UdgX excises uracil from uracil-containing DNA to concurrently form a covalent bond with the resulting AP-DNA. Structurally, UdgX is highly similar to family-4 UDGs (F4-UDGs). However, UdgX is unique in possessing a flexible R-loop (105KRRIH109). Our earlier studies allowed us to propose a reaction mechanism of UdgX, which involves the formation of a covalent bond between H109 of UdgX with the C1′ position of the target deoxyribose sugar concurrently with the uracil excision from this site in DNA.

Substitutions of His109 in MsmUdgX with Ser, Gly, Ala, Gln, Cys and Lys showed the loss of its covalent complex formation with DNA but gained canonical UDG activities. However, H109 substitutions by Gln or Lys, showed poor activity. Both Cys and Ala mutations of H109 showed intermediate Kcat/Km values. Further, the overlay of all the structures of UdgX H109 mutants showed that the overall structures are very well conserved with a Cα RMSD of ca 0.2 Å. As anticipated, we note a clear difference in the sizes of the active site cavities in the various mutants. When we arranged the mutants in the order of increasing cavity sizes (left), we noted that the canonical UDG activity of the mutants increased with their increasing cavity sizes to begin with and then with a further increase in the cavity size, the UDG activity declined (right). It suggested that the initial increase in UDG activity (H109K to H109Q to H109G) occurred because of the efficiency with which the water molecule could be localized to make a nucleophilic attack on the C1′ position. However, a further increase in the cavity size (H109S to H109C to H109A) perhaps destabilizes the bound water, thereby decreasing the UDG activity.

> AGAQDFVPHTADLAELAAAAGECRGCGLYRDATQAVFGAGGRSARIMMIGEQPGDKEDLAGLPFVGPAGRLLDRALEAADIDRDALYVTNAVKHFKFTRAAGGKRRICKTPSRTEVVACRPWLIAEMTSVEPDVVVLLGATAAKALLGNDFRVTQHRGEVLHVDDVPGDPALVATVHPSSLLRGPKEERESAFAGLVDDLRVAADVR>LIKSDQVNGVLVLSLLDKIIGAVDQIQLTQAQLEERQAEMEGAVQSIQGELSKLGKAHATTSNTVSKLLE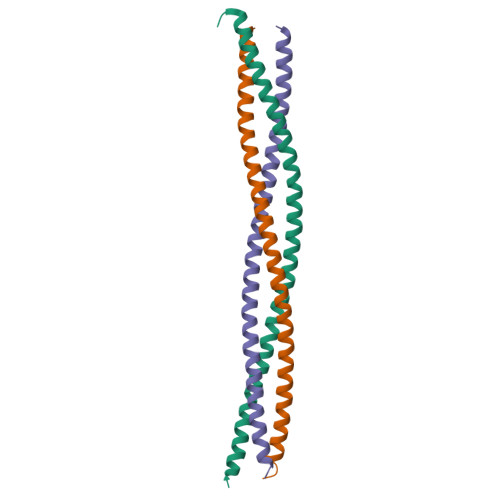KVRKVSVNVKTVRGSLERQAGQIKKLEVNEAELLRRRNFKV[3x]>MKVYLRKIDNQILHNKRISIKKGILEHFFDKANNQDEVDMSGILSNYNDKVSILLATDPRLGGGIKRIISAEVDKIKENR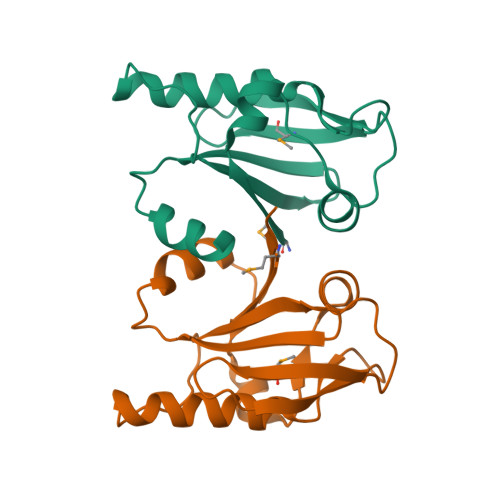LDYELKIDDILLFTYISYKKYTLEIILLADTRYNVLNGLINNSKHLLVFSENETRTLEHHHHHH[4x]> GAMDPEFTDEPIFGKKPRIEESITEDLSLADLMPRVKVQSVETVEGCTHEVALPAEEDYLPLKPRVGKAAKEYPFILDAFQREAIQCVDNNQSVL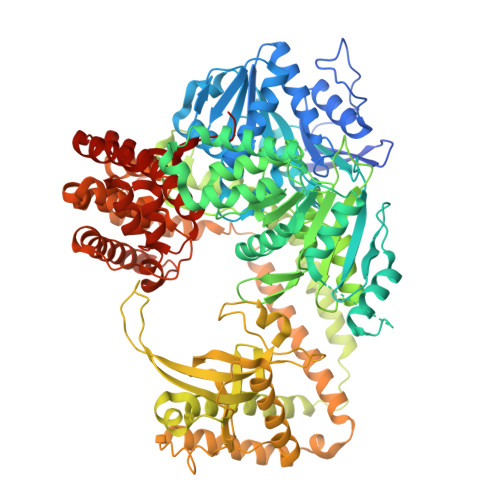VSAHTSAGKTVCAEYAIALALREKQRVIFTSPIKALSNQKYREMYEEFQDVGLMTGDVTINPTASCLVMTTEILRSMLYRGSEVMREVAWVIFDEIHYMRDSERGVVWEETIILLPDNVHYVFLSATIPNARQFAEWICHLHKQPCHVIYTDYRPTPLQHYIFPAGGDGLHLVVDENGDFREDNFNTAMQVLRDAGDLAKGDQKGRKGGTKGPSNVFKIVKMIMERNFQPVIIFSFSKKDCEAYALQMTKLDFNTDEEKKMVEEVFSNAIDCLSDEDKKLPQVEHVLPLLKRGIGIHHGGLLPILKETIEILFSEGLIKALFATETFAMGINMPARTVLFTNARKFDGKDFRWISSGEYIQMSGRAGRRGMDDRGIVILMVDEKMSPTIGKQLLKGSADPLNSAFHLTYNMVLNLLRVEEINPEYMLEKSFYQFQHYRAIPGVVEKVKNSEEQYNKIVIPNEESVVIYYKIRQQLAKLGKEIEEYIHKPKYCLPFLQPGRLVKVKNEGDDFGWGVVVNFSKKSNVKPNSGELDPLYVVEVLLRCSKESLKNSATEAAKPAKPDEKGEMQVVPVLVHLLSAISSVRLYIPKDLRPVDNRQSVLKSIQEVQKRFPDGIPLLDPIDDMGIQDQGLKKVIQKVEAFEHRMYSHPLHNDPNLETVYTLCEKKAQIAIDIKSAKRELKKARTVLQMDELKCRKRVLRRLGFATSSDVIEMKGRVACEISSADELLLTEMMFNGLFNDLSAEQATALLSCFVFQENSSEMPKLTEQLAGPLRQMQECAKRIAKVSAEAKLEIDEETYLSSFKPHLMDVVYTWATGATFAHICKMTDVFEGSIIRCMRRLEELLRQMCQAAKAIGNTELENKFAEGITKIKRDIVFAASLYL N-cyclopentyl-2-[(11,15-dimethyl-10-oxo-8-oxa-2,11,15,19,21,23-hexazatetracyclo[15.6.1.13,7.020,24]pentacosa-1(23),3(25),4,6,17,20(24),21-heptaen-6-yl)oxy]acetamide   | C27 H35 N7 O4 | 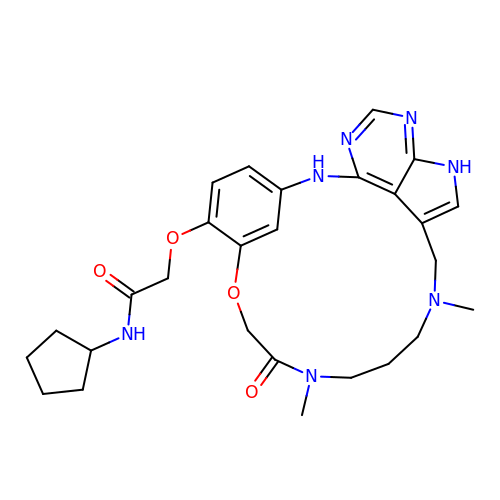MUBFRUUNEUDLMA-UHFFFAOYSA-N>GAMDAAVVVMPGTAAAPLPAIDVDAPFLNPKKQKAAELKEKIKISHDVTLFRFGLEHDEQLLGLPTGKHMLIRKKVTNAEGDEEVVMRAYTPTTANETRGHFDLVVKIYKANVHPKFPEGGKFSQI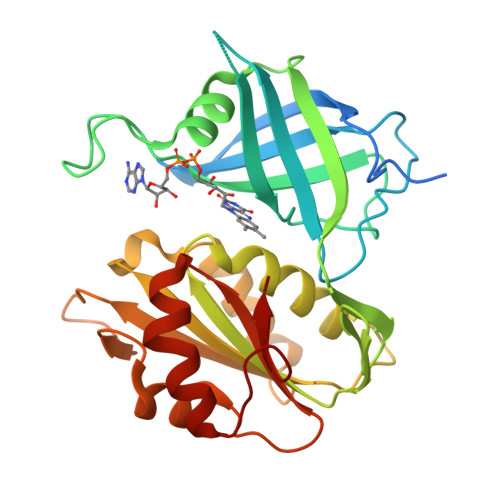LEALEVGDTVEVKGPIGHFHYDRPGHYKNHKLESEVKRINMIAGGTGLTPMYQVMKAILSNPSDLTEIRLLYANQTEADILLRPELEALAKSHPDRVKIHYTVDRPTPGWKYSSGFIDLDMCERALFRYEPGTISVLCGPPPMLKFACHPNLEKMGFEKGVTSIEF[2x]> AESTTLETIEIHPITFPPEVLARISPELSLQRHLSLGIRPCLRKYEEFRD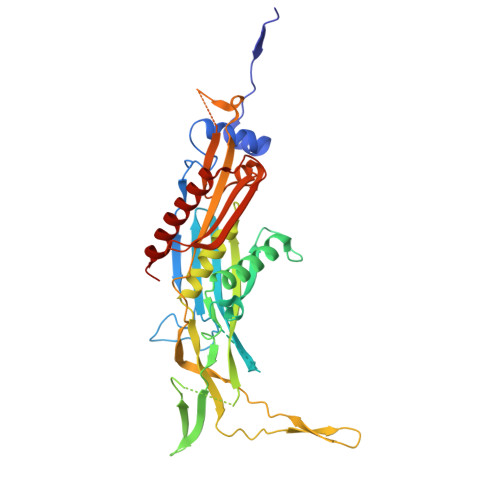VAIENNTLSRYADAGNIDTKNNILGSNVLKSGKTIVITSITGGIIEETSASIKDLDDFGEEELFEVTKEEDIIANYASVYPVVEVERGRVGACTDEEMTISQKLHDSILHSRILPKKALKVKAGVRSANEDGTFSVLYPDELEDDTLNETNLKMKRKWSYVLYAKIVVLSRTGPVFDLCWNSLMYALQSVKLPRAFIDERASDLRMTIRTRGRSATIRETYEIICDQTKSVPLMINAKNIAFASNYGIVELDPECQLQNSDNSEEEEVDIDMDKLNTVLIADLDTEAEETSIHSTISILAAPSGNYKQLTLMGGGAKITPEMIKRSLLLSRVRADDLSTRFNI>GHMNVKLKVFHAGSLTEPMKAFKRAFEEKHPNVEVQTEAAGSAATIRKVTELGRKADVIATADYTLIQKMMYPEFAN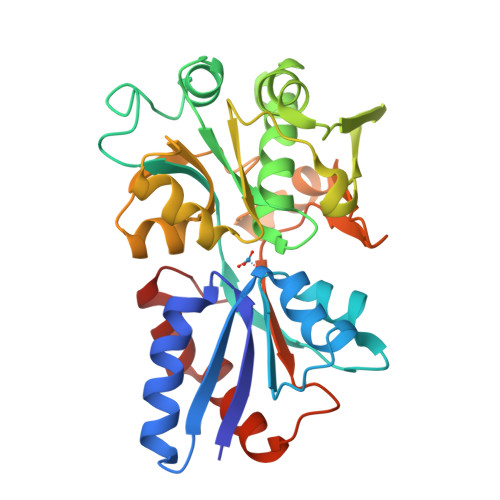WTIMFAKNQIVLAYRNDSRYADEINSQNWYEILKRPDVRFGFSNPNDDPCGYRSLMAIQLAELYYNDPTIFDELVAKNSNLRFSEDNGSYVLRMPSSERIEINKSKIMIRSMEMELIHLVESGELDYFFIYKSVAKQHGFNFVELPVEIDLSSPDYAELYSKVKVVLANGKEVTGKPIVYGITIPKNAENRELAVEFVKLVISEEGQEILRELGQEPL[2x]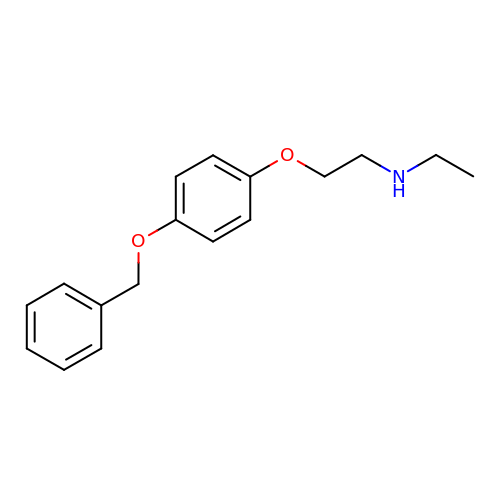2-[4-(benzyloxy)phenoxy]-N-ethylethan-1-amine | C17 H21 N O2 | DLYGRQINMSKZKQ-UHFFFAOYSA-N>[4x]TLKGKTALVTGSTSGIGLGIAQVLARAGANIVLNGFGDPAPALAEIARHGVKAVHHP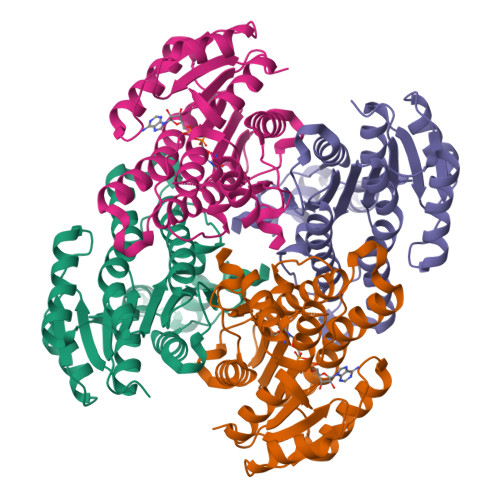ADLSDVAQIEALFALAEREFGGVDILVNNAGIQHVAPVEQFPLESWDKIIALNLSAVFHGTRLALPGMRARNWGRIINIASVHGLVGSTGKAAYVAAKHGVVGLTKVVGLETATSNVTCNAICPGWVLTPLVQKQIDDRAANGGDPLQAQHDLLAEKQPSLAFVTPEHLGELVLFLCSEAGSQVRGAAWNVDGGWLAQ(2Z,5R)-3-(3-chlorobenzyl)-2-imino-5-methyl-5-(2-methylpropyl)imidazolidin-4-one 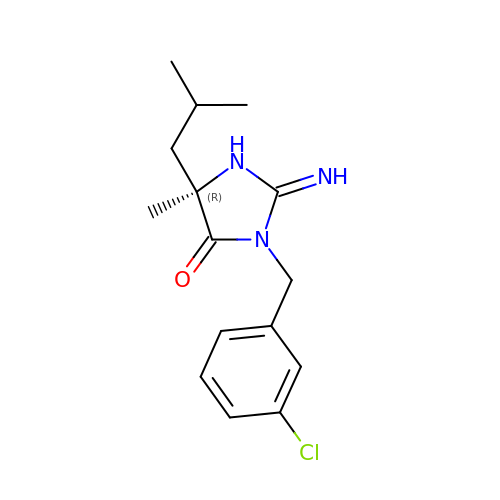| C15 H20 Cl N3 O | SMHLWQCDIJPLEC-OAHLLOKOSA-N>MARRLPKPTLQGRLEADFPDSPLLPKFQELNQNNLPNDVFREAQRSYLVFLTSQFCYEEYVQRTFGVPRRQRAIDKRQRASVAGAGAHAHLGGSSATPVQQAQAAASAGTGALASSAPSTAVAQSATPSVSSSISSLRAATSGATAAASAAAAVDTGSGGGGQPHDTAPRGARKKQ[16x];>MKVQGSVDRRRLQRRIAGLLPPPARRLNISRGSEFTRDVRGLVEEHAQASSLSAAAVWRAGLLAPGEVAVAGGGSGGGSFSWSGWRPPVFGDFLIHASSFNNAEATGTPLFQFKQSDPFSGVDAVFTPLSLFILMNHGRGVAARVEAGGGLTRMANLLYDSPATLADLVPDFGRLVADRRFHNFITPVGPLVENIKSTYLNKITTVVHGPVVSKAIPRSTVKVTVPQEAFVDLDAWLSGGAGGGGGVCFVGGLGLQPCPADARLYVALTYEEAGPRFTFFQSSRGHCQIMNILRIYYSPSIMHRYAVVQPLHIEELTFGAVACLGTFSATDGWRRSAFNYRGSSLPVVEIDSFYSNVSDWEVIL[5x];>[10x]MDLKVVVSLSSRLYTDEIAKMQQRIGCILPLASTHGTQNVQGLGLGQVYSLETVPDYVSMYNYLSDCTLAVLDEVSVDSLILTKIVPGQTYAIKNKYQPFFQWHGTGSLSVMPPVFGREHATVKLESNDVDIVFPMVLPTPIAEEVLQKILLFNVYSRVVMQAPGNADMLDVHMHLGSVSYLGHHYELALPEVPGPLGLALLDNLSLYFCIMVTLLPRASMRLVRGLIRHEHHDLLNLFQEMVPDEIARIDLDDLSVADDLSRMRVMMTYLQSLASLFNLGPRLATAAYSQETLTATCWLR;>MASNEGVENRPFPYLTVDADLLSNLRQSAAEGLFHSFDLLVGKDAREAGIKFEVLLGVYTNAIQYVRFLETALAVSCVNTEFKDLSRMTDGKIQFRISVPTIAHGDGRRPSKQRTFIVVKNCHKHHISTEMELSMLDLEILHSIPETPVEYAEYVGAVKTVASALQFGVDALERGLINTVLSVKLRHAPPMFILQTLADPTFTERGFSKTVKSDLIAMFKRHLLEHSFFLDRAENMGSGFSQYVRSRLSEMVAAVSGESVLKGVSTYTTAKGGEPVGGVFIVTDNVLRQLLTFLGEEADNQIMGPSSYASFVVRGENLVTAVSYGRVMRTFEHFMARIVDSPEKAGSTKSDLPAVAAGVEDQPRVPISAAVIKLGNHAVAVESLQKMYNDTQSPYPLNRRMQYSYYFPVGLFMPNPKYTTSAAIKMLDNPTQQLPVEAWIVNKNNLLLAFNLQNALKVLCHPRLHTPAHTLNSLNAAPAPRDRRETYSLQHRRPNHMNVLVIVDEFYDNKYAAPVTDIALKCGLPTEDFLHPSNYDLLRLELHPLYDIYIGRDAGERARHRAVHRLMVGNLPTPLAPAAFQEARGQQFETATSLAHVVDQAVIETVQDTAYDTAYPAFFYVVEAMIHGFEEKFVMNVPLVSLCINTYWERSGRLAFVNSFSMIKFICRHLGNNAISKEAYSMYRKIYGELIALEQALMRLAGSDVVGDESVGQYVCALLDPNLLPPVAYTDIFTHLLTVSDRAPQIIIGNEVYADTLAAPQFIERVGNMDEMAAQFVALYGYRVNGDHDHDFRLHLGPYVDEGHADVLEKIFYYVFLPTCTNAHMCGLGVDFQHVAQTLAYNGPAFSHHFTRDEDILDNLENGTLRDLLEISDLRPTVGMIRDLSASFMTCPTFTRAVRVSVDNDVTQQLAPNPADKRTEQTVLVNGLVAFAFSERTRAVTQCLFHAIPFHMFYGDPRVAATMHQDVATFVMRNPQQRAVEAFNRPEQLFAEYREWHRSPMGKYAAECLPSLVSISGMTAMHIKMSPMAYIAQAKLKIHPGVAMTVVRTDEILSENILFSSRASTSMFIGTPNVSRREARVDAVTFEVHHEMASIDTGLSYSSTMTPARVAAITTDMGIHTQDFFSVFPAEAFGNQQVNDYIKAKVGAQRNGTLLRDPRTYLAGMTNVNGAPGLCHGQQATCEIIVTPVTADVAYFQKSNSPRGRAACVVSCENYNQEVAEGLIYDHSRPDAAYEYRSTVNPWASQLGSLGDIMYNSSYRQTAVPGLYSPCRAFFNKEELLRNNRGLYNMVNEYSQRLGGHPATSNTEVQFVVIAGTDVFLEQPCSFLQEAFPALSASSRALIDEFMSVKQTHAPIHYGHYIIEEVAPVRRILKFGNKVVF[16x]

Epstein-Bar virus (EBV), a member of the subfamily gammaherpesviruses that also includes the Kaposi Sarcoma-associated herpesvirus (KSHV),2,3 is the first identified oncovirus. Similar to other members of the family herpesviridae, EBV has a characteristic three-layer configuration: the outer lipid bilayer envelope containing viral glycoproteins responsible for host recognizing and membrane fusion, the inner pseudo-icosahedral nucleocapsid enclosing a 172-kb double-strand DNA (dsDNA) genome and the middle pleomorphic tegument compartment fulfilled with 20–40 different viral proteins. All herpesvirus capsid shell consists of 4 abundant proteins: the major capsid proteins (MCP) constituting the basic capsid skeleton through forming 150 hexons and 11 pentons, the small capsid proteins (SCP) binding to the tops of hexon MCPs or both hexon and penton MCPs, and the Tri1 and Tri2 forming the heterotrimeric triplexes to plug the large holes on the capsid floor. Once the viral dsDNA genome enters the procapsid shell through the portal that is located at a unique 5-fold vertex of the icosahedral capsid, the viral nucleocapsid is joined by the capsid-associated tegument complexes (CATCs).

We obtained an icosahedral reconstruction at a resolution of 4.1 Å from 32,721 particles, which, complemented by a 3.5 Å structure of the penton-vertex region through sub-particle classification and refinement, allowed us to build an ab initio atomic model for the viral capsid, including 16 copies of MCPs, 16 copies of SCPs, 5 copies of the triplex monomer proteins (Tri1) and 10 copies of triplex dimer proteins (Tri2). As observed in other herpesviruses, the EBV MCPs are extensively interconnected through three types of interactions between the floor regions of MCPs. The type 1 interaction is an intracapsomer β-augmentation between two neighboring MCPs within a hexon or penton capsomer. The type 2 interaction is an intercapsomer and quasiequivalent interaction between two pairs of α-helices from the dimerization domains of MCPs across local 2-fold axes. The type 3 interaction is built upon and further strengthens the type 1 interaction. Each of the EBV SCPs binds the tops of two adjacent MCPs both in a hexon and in the penton. The triplexes, heterotrimers of one Tri1 molecule and two Tri2 conformers (Tri2A and Tri2B), plug the large holes on the capsid floor. The triplex is then anchored to the capsid by the N-anchor of Tri1 that traverses the capsid floor, extends along the capsid inner surface and folds into a tripod of helices. There are five types of triplexes, Ta to Te, located at local 3-fold axes. The triplexes Tb to Te adopt a similar structure, whereas the Ta has a unique conformation with its N-anchor rotated ~120° counterclockwise compared to the others.> SDGETSVQPMMTKIKTVLKSRGRPPTEPLPDGWIMTFHNSGVPVYLHRESRVVTWSRPYFL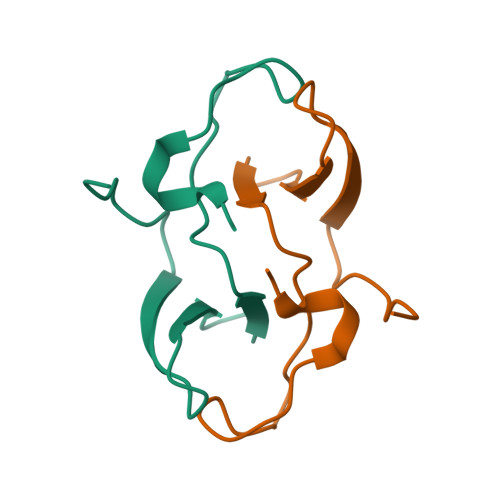GTGSIRKHDPPLSSIPCL> GSAENESTPIQQLLEHFLRQLQRKDPHGFFAFPVTDAIAPGYSMIIKHPMDFGTMKDKIVANEYKSVTEFKADFKLMCDNAMTYNRPDTVYYKLAKKILHAGFKMMSK;> SGRGXG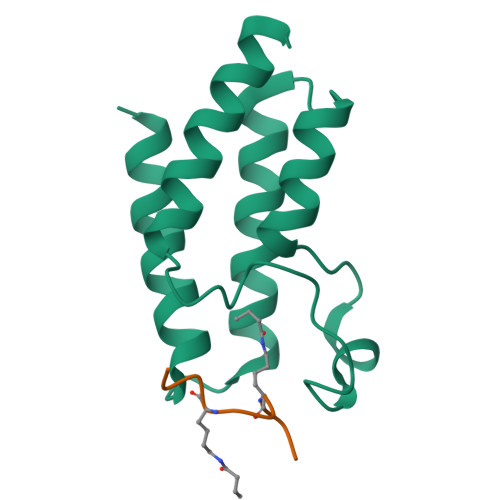GXGLG>[2x]GAMALPQGDEIAYVPIGSITLESGAVIDDVTIAVQSWGELSPRRDNV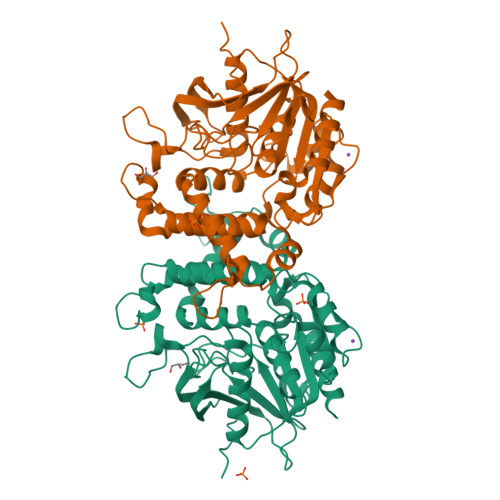VFVCHALTADSHVVGPAGPDHITGGWWEGIIGPGAAIDTDHWCAVATNVLGGCRGTTGPTSLARDGKPWGSRFPEVSVRDQVNADVAALAQLGITEVAAVVGGSMGGARALEWAVMHPDAVRAALVLAVGARATGDQIGTQSTQIAAIQTDPDWQGGDYHGSGRSPGKGLNLARRIAHLTYRGEVELDTRFGNDPQVGPDGPEDPWADGRYAVQSYLEHQGNKFVRRFDAGSYVILTESLNRHDVGRGRGGVEKALRGCPVPVVVGGITSDRLYPLRLQEELADLLPGCTGLRVVESVHGHDAFLIEFDAVSELVRETLALAK>MA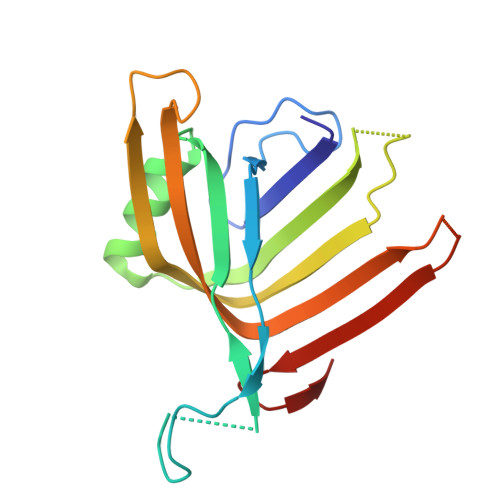YDIFLKIDGIDGESMDDKHKNEIEVLSWRWNIHQESTMHAGSGLGSGKVSVTNLDFDHYIDRASPNLFKYCASGKHIPQAILVMRKAGGNPLEYLKYTFTDLIVAVVSPSGSHDGEIASRETVELSFSTVKQEYVVQNQQGGSGGTITAGYDFKANKEI[3x]>XLA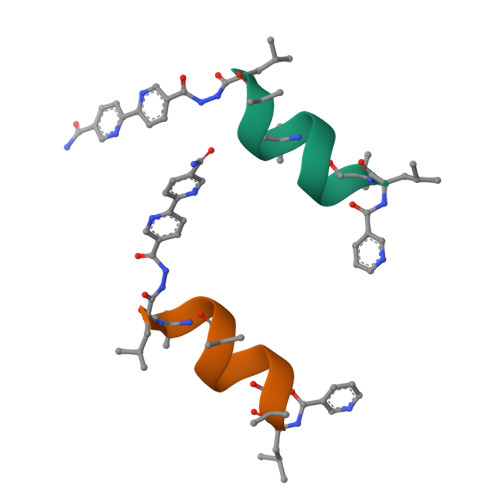ACLAQALX[4x]>[4x]TSSANEDMPVE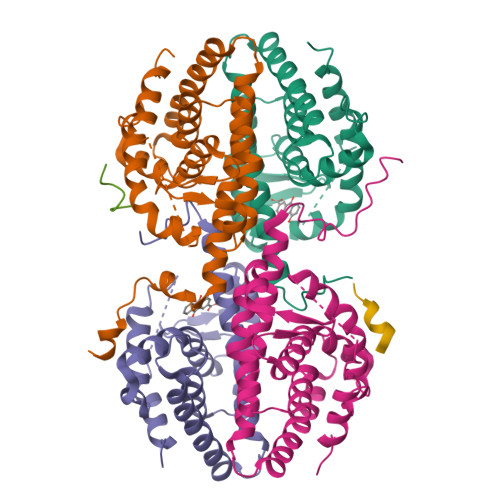RILEAELAVEPKTETYVEANMGLNPSSPNDPVTNICQAADKQLFTLVEWAKRIPHFSELPLDDQVILLRAGWNELLIASFSHRSIAVKDGILLATGLHVHRNSAHSAGVGAIFDRVLTELVSKMRDMQMDKTELGCLRAIVLFNPDSKGLSNPAEVEALREKVYASLEAYCKHKYPEQPGRFAKLLLRLPALRSIGLKCLEHLFFFKLIGDTPIDTFLMEMLEAPHQMT;>[2x]TNMGLEAIIRKALMGK>[4x]MDQFREIGEVLGS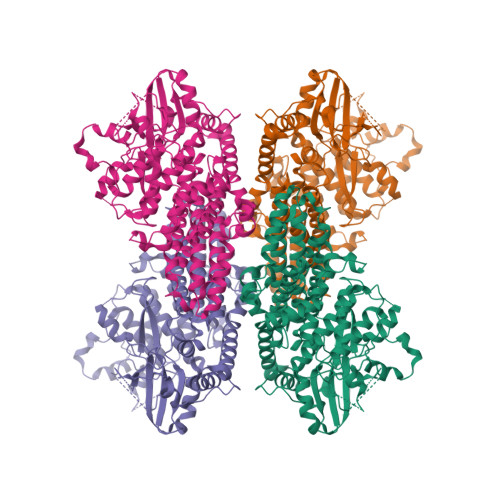IRALMVFKDSIQINQRQCSLLLDLFTAAYESISVSMRSNLRFKEKNTKWKILEQPLRELLWVVREGEAYVRMSLEPKLGFWAKAIVLHSNRDCTELHIHNLLSCLPIIVEAIETASEVSGWDEEEMSKKRLVHSNKYMKQWNDSQMFTWKFGREYLVTEDFCNRFESAWTEDRWILIKELQEKKQSGSSKHERKMADFLLKHLGDGNESPKLFPSSLLDNTKDYQVKKRLGNGSQYKEITWLGESFALRHFFGDIDALLPQITPLLSLSHPNIVYYLCGFTDEEKKECFLVMELMRKTLGMHIKEVCGPRKKNTLSLPVAVDLMLQIALGMEYLHSKRIYHGELNPSNILVKPRSNQSGDGYLLGKIFGFGLNSVKGFSSKSASLTSQNENFPFIWYSPEVLEEQEQSGTAGSLKYSDKSDVYSFGMVSFELLTGKVPFEDSHLQGDKMSRNIRAGERPLFPFNSPKFITNLTKRCWHADPNQRPTFSSISRILRYIKRFLALNPECYSSSQQDPSIAPTVDYCEIETKLLQKLSWESTELTKVSQVPFQMFAYRVVERAKTCEKDNLREPSESGSEWASCSEDEGGAGSDEQLSYAKERRLSCSSNDVGMSKKQVSNLLKRASSLKPIQKPAFGFCSGTTPRGRSRHPPLSPCGGQSMRANSESQLILISPRIRRSNSGHASDSELS With the new chain-extended nucleoside oligophosphates in hand, we go on to investigate in detail their interaction with ribonuclease A, a model protein containing a polycationic active site and for which X-ray crystal structures are relatively straightforward to obtain. Thus, we go on to investigate in detail the interaction of the polyanionic constructs with ribonuclease A, a model protein containing a polycationic active site and for which X-ray crystal structures are relatively straightforward to obtain. This work presents a combined experimental and quantum chemical approach to understanding the interactions of RNase A with the new nucleoside hexa- and heptaphosphate constructs. To better comprehend RNase A and nucleoside oligophosphate interactions, we examine the correlation between the experimental and calculated protein–ligand interactions by combining efforts in crystallographic and computational investigations in the present work. The combination of the CCSD(T) approach with the appropriate energy decomposition scheme enables deciphering the influence of the oligophosphate chain length and of individual polypeptide and nucleoside residues on ligand binding.

Here, we demonstrate by extending adenosine monophosphate (AMP) and uridine monophosphate (UMP) to their corresponding nucleoside hexaphosphates, while adenosine diphosphate (ADP) and uridine diphosphate (UDP) are phosphate chain-extended to the corresponding nucleoside heptaphosphates. In the presence of Mo(NCMe)3(CO)3,35 [PPN]2[TBA]1 readily reacted with anhydrous NMPs and NDPs, yielding the corresponding hexa- and heptaphosphates after subsequent hydrolysis. Anion-exchange HPLC purification of the resulting compounds provided the ammonium salts of adenosine/uridine hexaphosphates (50% yield for p6A and 29% for p6U) and adenosine/uridine heptaphosphates (24% yield for p7A and 17% for p7U). This result represents the first direct chemical syntheses of nucleoside-5′-hexa- and -heptaphosphates. Additionally, we found that the hydrolytic ring-opening process exhibits less selectivity when leading to the nucleoside heptaphosphates as compared with that leading to the nucleoside hexaphosphates, with observed formation of pentametaphosphate and NDPs. Aqueous solutions of the purified nucleoside hexa- and heptaphosphates were observed to be stable for at least a week, as confirmed by 31P{1H} NMR spectroscopy.

>KETAAAKFERQHMDSSTSAASSSNYCNQMMKSRNLTKDRCKPVNTFVHESLADVQAVCSQKNVACKNGQTNCYQSYSTMSITDCRETGSSKYPNCAYKTTQANKHIIVACEGNPYVPVHFDASV[2x]> MVQISEVRGNTRDHRTAAHTHIKGLGLNSSGIAEKQAAGFVGQCAAREA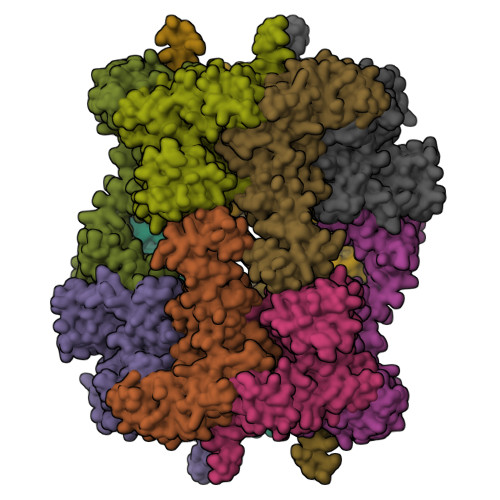CGVVVDLIKAHKMAGRGVLLAGGPGTGKTALALAISQELGTKIPFCPITGSEIYSTEVKKTEVLMENFRRAIGLRVRETKDVYEGEVTEMTPEEAENPLGGYGKTISTLLIGLKSARGQKKLRLDPSIYEAIQKERVQVGDVIYIETNTGACKRVGRSDAYATEFDLEAEEYVPIPKGEVHKKKEIVQDVTLHDLDVANARPQGGQDIISMMGQLMKPKMTEITDKLRMEINKVVQKYINQGVAELIPGVLFIDEAHMLDIECFTYLNKALESPIAPIVVLASNRGIATIRGADDLKAAHGIPPDFLQRLLIIPTHPYEPDEIRRIVRIRAQTEGVQLTDAAVDRVAEHGVRISLRYCLQLLAPASILARVNGRTQVDVQDIAEAEELFLDARRSANILTSTGESGGLHGFIS;> MGSSHHHHHHHHSSGLEVLFQGPGSMAAPLVTSVTETKELRGLNLIAAHSHIRGLGVDADTLEPRPSSQGLVGQEKARKAAAVVLEMIKQGKIAGRAVLIAGPPSTGKTAIAMGMAQSLGQDVPFTTLAASEIFSLEMSKTEALTQAFRKSIGVRIKEESEIMEGEVVEIQIDRSVTGGAKQGKLTIKTTDMEAIYDMGSKMIDAMTKERVMAGDIISIDKSSGKITKLGRSYARSRDYDAMGVDTKFLQCPEGELQKRKEVVHTVSLHEIDVINSRTQGFLALFSGDTGEIRSEIRDQINTKVAEWKEEGKAEIVPGVLFIDEVHMLDIECFSYINRALESDLAPIVIMASNRGVSRIRGTDYKSPHGLPLDFLDRVVIINTHPYTPDELRQILSIRAQEEEVDLTPDALALLTKIGQEAGLRYASNLITTSQLIAAKRRAKQVGVEDVQRSFKLFYDPARSVRFVQESEKRLIGNDGVVDFSYQGAAEAAAPTLPAAAPVDPVGGEKMDMS The Mex67–Mtr2 complex (NXF1–NXT1 in metazoans and small bristles in Drosophila melanogastor) is the principal mRNA-export factor in Sacccharomyces cerevisiae. Mex67/NXF1 is a modular protein constructed from four domains: an RNA-recognition motif (RRM) domain, a leucine-rich repeat (LRR) domain, a nuclear transport factor 2-like (NTF2L) domain and an ubiquitin-associated (UBA) domain. Mtr2 is a ∼15–20 kDa protein that also has an NTF2-like fold and forms a tight heterodimeric complex with the Mex67 NTF2L domain.

The ctMex67NTF2L and ctMtr2 chains interacted through their highly curved β-sheets in a pseudo-twofold-symmetric manner in the 2.9 Å resolution crystal structure, similar to that observed in the analogous complexes from H. sapiens and S. cerevisiae. In the complex, ctMtr2 was not altered when compared with the isolated structure, with a Cα r.m.s.d. of 0.38 Å over 148 residues. More recently, the NTF2L domain and Mtr2 have also been implicated in binding ribosomal subunits and rRNA, whereby in S. cerevisiae specific long internal loops may be involved in direct RNA binding as well as domain organization to form a continuous RNA-binding platform with the RRM and LRR domains. There was clear density for these loops in the ctMex67NTF2L–Mtr2 crystal structure, but as in hsNXF1NTF2L–NXT1 they did not form an extended surface, suggesting that ctMex67–Mtr2 may not be involved in ribosomal export in C. thermophilum in the quite same way as in S. cerevisiae. The position of the pre-α1 loop, which has been implicated in the spatial arrangement of the Mex67 domains in S. cerevisiae, occupied a similar position in ctMex67NTF2L to that observed in S. cerevisiae and H. sapiens. In particular, Leu368 was buried in a hydrophobic pocket present in ctMtr2. Notably, Leu368 was positioned in a structurally equivalent position to scMex67Leu263 and hsNXF1Leu370, indicating that the NTF2L pre-α1 loop position may be conserved across species. C. thermophilum Mex67–Mtr2 retained features found in both S. cerevisiae and H. sapiens and conserved the hydrophobic pocket identified as the nucleoporin-binding site found in NTF2L domains from other organisms.

> GSHHHHHHSQDPMPTPLPQLPSNVRDGENNVASTFLQAFFQLWDHDRLTLIPQFYDSETTFSVVFATDSPQDPASSSCSKFSRNLNILSPRHPSTLQRLFVGSNLIADLWKVLPATRHPSLDQTSQWLIDCHTFPHLADPTGMAPYAMGLMINVNGQCEEADISQNLYGTRTFSRCFILGPSKPGAPHPYRVLSDQLTLHTWKPQPAPQVGTV;> MLSRRYAAKSFVEWYYRQINENKPVASGYVNNNATYTKAGHPPADITINGRVVATPEEWDTMLKEQRAQHNTSSSSTLPIGRKPVRYDVDCFDVHVINADYRFAAPQRMIEQHAPTDGVRMMMALTVSGSVYFGASPRSTDDYVIKQHFNDVFILVPNWDVLEKPGARSARKYLIASHKYRAY Meromycolate extension acyl carrier protein (AcpM) serves as the carrier of fatty acyl chain shuttling among the individual FAS-II components during the progression of fatty acid elongation. In this study, MSMEG_5634 in Mycobacterium smegmatis was identified as a novel acyl-AcpM-binding protein. MSMEG_5634 and its homologous proteins are highly conserved among mycobacteria and belong to the SRPBCC (START/RHOs_alpha_C/PITPs/Bet v1/CoxG/CalC) superfamily, containing a START domain that functions as a lipid-binding domain involved in eukaryotic signal transduction as well as a cyclase/aromatase domain for the biosynthesis of polyketide antibiotics in Actinomycetes. MSMEG_5634 can transport acyl-AcpM away from FAS-II by forming the MSMEG_5634/acyl-AcpM complex and contributes to intrinsic sensitivity to FAS-II inhibitors.

The structure of MSMEG_5634 was solved at 1.9 Å resolution. MSMEG_5634 has a helix-grip structure that contains seven-stranded antiparallel β-sheets (named β1 to β7) and four α-helices (α1 to α4). α1 and α2 are two short consecutive helices located between β1 and β2, and α3 is also a short α-helix which is followed by the long C-terminal helix α4. The seven-stranded antiparallel β-sheets and the long C-terminal α-helix α4 together fold into a barrel, with a deep hydrophobic pocket wrapped in the middle of the barrel. The first two short helices α1 and α2 fold into a V-shaped structure that seals the bottom of the pocket. A clear linear electron density was observed inserted into the pocket of MSMEG_5634, which might be a chain of a fatty acid based on its shape, indicating that MSMEG_5634 may bind fatty acid chain-containing substrate. In the refined structure of the MSMEG_5634 protein expressed and purified from E. coli, there was a linear electron density, which might be a chain of fatty acid inserted into the pocket of MSMEG_5634. The overall structure of MSMEG_5634 is similar to that of the TcmN polyketide cyclase/aromatase domain but with differences in the conformation of proposed active site residues. According to the protein sequence and structure, the corresponding residues of MSMEG_5634 are Tyr-27, Arg-63, -65, and -84, but the side chains of Arg-63, -65, and -84 all point to the outside of the pocket. Third, the ligand-binding pocket of MSMEG_5634 is more hydrophobic than the pocket of TcmN ARO/CYC. The interaction between MSMEG_5634 and acyl-AcpM was disrupted by the substitution mutation of W30A in helix α2, which formed a helix–loop–helix motif together with the α1 helix at the bottom of the pocket.

> SMAKLSVSVEVPLPPEQAWEYASDLSRYHEWLSIHRAWRSKLPETLEKGTVIESIVEVKGMLNRVRWTLVHYKPPQALTLNGDGRGGVKVKLIGKIKPTDNGATVGFDLHLGGPALFGPIGMVVAAALKSDIQESLNRFKQLYAPSAT> YVP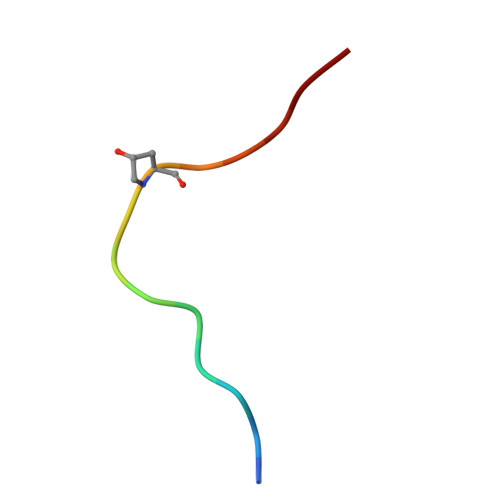VPASGPSRKHN> GSHMMPITINNFRYSDPVNNDTIIMMEPPYCKGLDIYYKAFKITDRIWIVPERYEFGTKPEDFNPPSSLIEGASEYYDPNYLRTDSDKDRFLQTMVKLFNRIKNNVAGEALLDKIINAIPYLGNSYSLLDKFDTNSNSVSFNLLEQDPSGATTKSAMLTNLIIFGPGPVLNKNEVRGIVLRVDNKNYFPCRDGFGSIMQMAFCPEYVPTFDNVIENITSLTIGKSKYFQDPALLLMHELIHVLHGLYGMQVSSHEIIPSKQEIYMQHTYPISAEELFTFGGQDANLISIDIKNDLYEKTLNDYKAIANKLSQVTSCNDPNIDIDSYKQIYQQKYQFDKDSNGQYIVNEDKFQILYNSIMYGFTEVELGKKFNIKTRLSYFSMNHDPVKIPNLLDDTIYNDTEGFNIESKDLKSEYKGQNMRVNTNA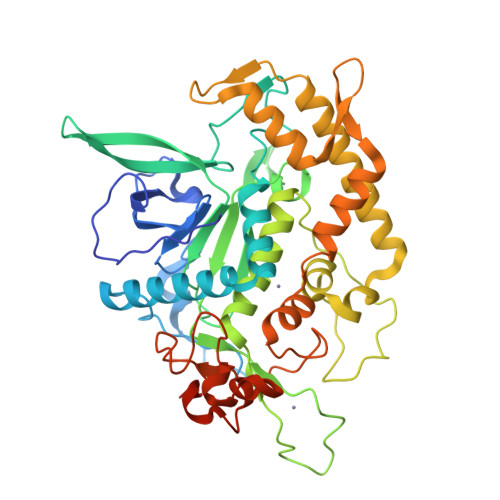FRNVDGSGLVSKLIGLCKKII> SAAGKDCITIHSATFAWSQESPPCLHRINLTVPQGCLLAVVGPVGAGKSSLLSALLGELSKVE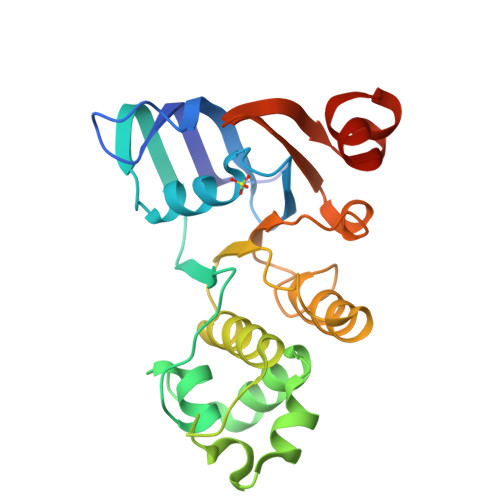GFVSIEGAVAYVPQEAWVQNTSVVENVCFGQELDPPWLERVLEACALQPDVDSFPEGIHTSIGEQGMNLSGGQKQRLSLARAVYRKAAVYLLDDPLAALDAHVGQHVFNQVIGPGGLLQGTTRILVTAALHILPQADWIIVLANGAIAEMGSYQELLQRKGALVCLLDQARQPGD>[4x]MEERNDWHFNIGAMYEIENVEGYGEDMDGLAEPSVYFNAANGPWRIALAYYQEGPVDYSAGKRGTWFDRPELEVHYQFLENDDFSFGLTGGFRNYGYHYVDEPGKDTANMQRWKIAPDWDVKLTDDLRFNGWLSMYKFANDLNTTGYADTRVETETGLQYTFNETVALRVNYYLERGFNMDDSRNNGEFSTQEIRAYLPLTLGNHSVTPYTRI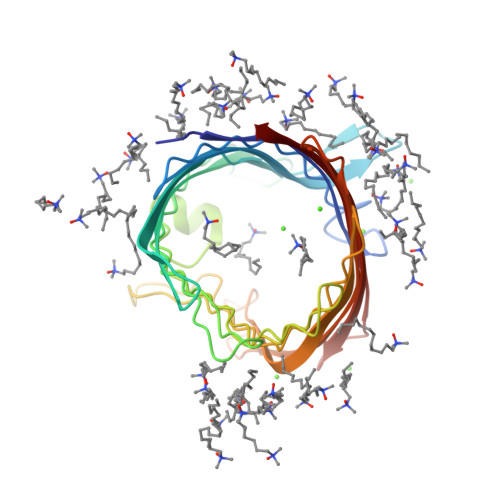GLDRWSNWDWQDDIEREGHDFNRVGLFYGYDFQNGLSVSLEYAFEWQDHDEGDSDKFHYAGVGVNYSF>MLWKK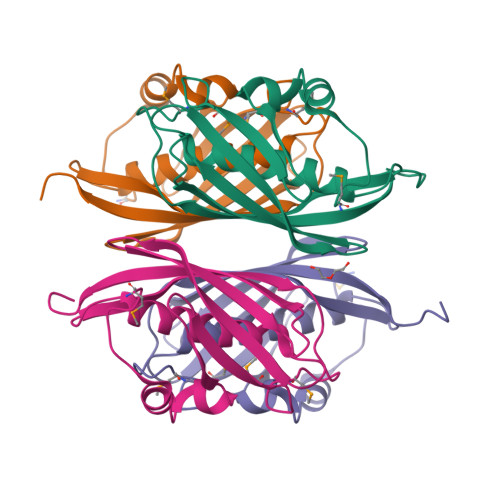TFTLENLNQLCSNSAVSHLGIEISAFGEDWIEATMPVDHRTMQPFGVLHGGVSVALAETIGSLAGSLCLEEGKTVVGLDINANHLRPVRSGKVTARATPINLGRNIQVWQIDIRTEENKLCCVSRLTLSVINLLEHHHHHH[4x]>MGSDKIHHHHHHMEVKIEKPTPEKLKELSVEKWPIWEKEVSEFDWYYDTNETCYILEGKVEVTTEDGKKYVIEKGDLVTFPKGLRCRWK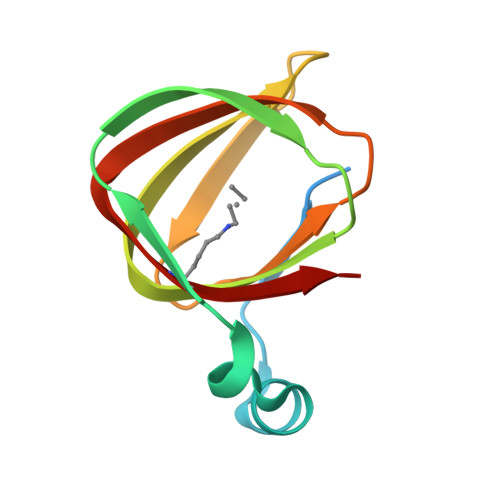VLEPVRKHYNLF[2x]>[4x]CTAITYVSKDHYFGRNFDYEISYNEVVTITPRNYKFSFREVGNLDHHFAIIGIAAGIADYPLYYDAINEKGLGMAGLNFSGYADYKKIEEGKENVSPFEFIPWVLGQCSTVDEAKKLLKNLNLVN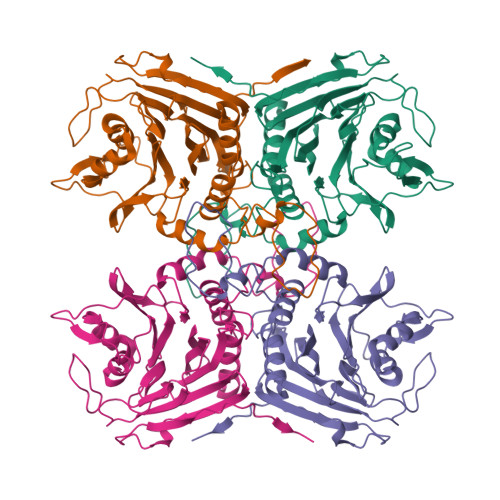INFSDELPLSPLHWLLADKEQSIVVESTKEGLRVFDNPVGVLTNNPTFDYQLFNLNNYRVLSTRTPKNNFSDQIELDIYSRGMGGIGLPGDLSSVSRFVKATFTKLNSVSRSSEYESISQFFHILSSVEQQKGLCDVGDEKYEYTIYSSCCNLEKGIYYYRTYDNSQITAVDMNKENLEKDSLIVYPMVETQQINYANLEHHHHHH> SQSYPKGSFHEGHINPFADVQWISRPFMKRNMPRDHHPLAKQHTSLKAVTMLDEESGNHWHVLDGKGRSVGGLAAQVVRLLQGKHRVD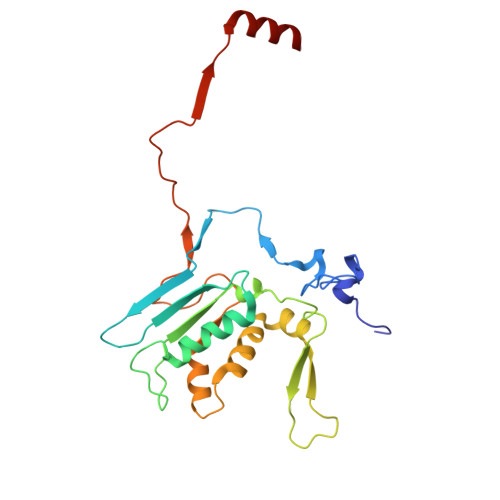FTPRTAAGDSVIVVNAIHLKMAGHTWDTKVYKFDRKTHPAGPKIITAKTIMARNPAMILNLAVKRMLPPNRLRPIMYRKLFVYAGALHPHWQVPQVIVPAKTPAEVSFLPFSVERADPVQAAARIAALG> GGELMIKSSNAFDVIELSSQIQRYASLSKINNRTNPILKDNKAKEFKDADLKWLKLENCPTAGDVPTTGNNNDLQDQFIACDADYRKGDLSYFGSQFEFSTYVHPSNPEIQRQIKQVVSYFQYRGMERAFIGDAAGYVISEAKKKGFSAQDYRIVLIEPDRVGYFESNAISYEEFIENPSARENFLLKATKDRTLALAVSLAQTGEIAMQRDGSVAFLEDSELCWDTAAGSAKSCLSVRYDTVGNKTELDLKQIDVVSAKGLSFESDGKTKTPVVSTYETFQDGGRAKTINAIECPTGLNNRFAAVVSSFSTAGQNANFSSESAKDSQGTTQKDGSKGPHALLSGISLNWTLTNKVW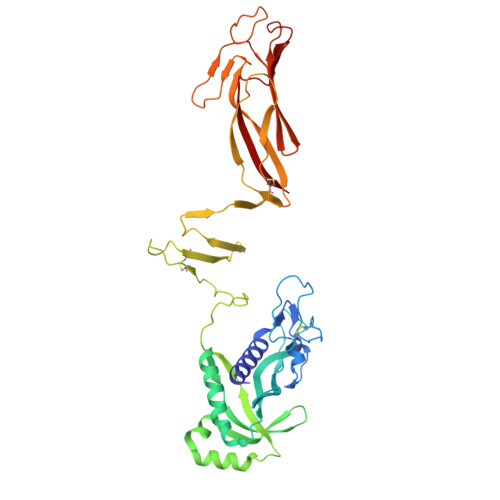DVTASIGIESGILPTSGIDSGSLLRNPKSLSFIAFQWCEN>[3x]PMFIVNTNVPRASVPDGF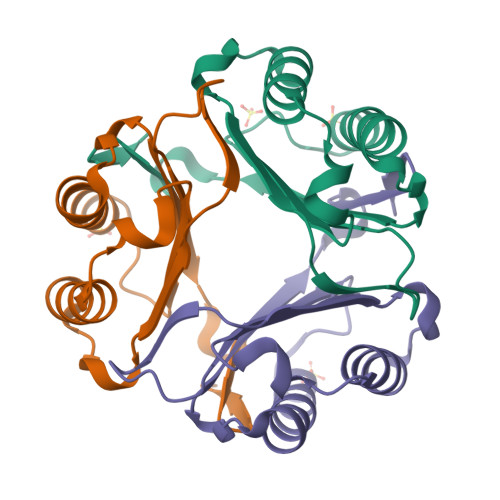LSELTQQLAQATGKPPQYIAVHVVPDQAMAFGGSSEPCALCSLHSIGKIGGAQNRSYSKLLCGLLAERLRISPDRVYINYYDMNAANVGWNNSTFA>MGLKALFFDVQGTLVDFYSTITREGEAFSAVRGFQADWTTVTEQWRAEYRSRLDQVIKGERPWTTTDRIYREALDGILANHPWGASLNSADRDELNSLWSKLIPWDDTAPGLARLRSKYITSTLSNGSMASVLRISKLGALPFDAILTAELVRSSKPDPKVYQLALDSVGIEAHQAMMVACHKYDLQAAKRLGFKVAFIARPFEFGPNKKVDTKPEQYFDYYANSVVELAGMLGALEHHHHHH[2x]

Microbial epoxide hydrolases, cis-epoxysuccinate hydrolases (CESHs), have been utilized for commercial production of enantiomerically pure L(+)- and D(−)-tartaric acids for decades. All these three CESH[L]s exhibit high sequence identity (>60%) with L-2-haloacid dehalogenases, which are members of the haloacid dehalogenase (HAD)-like superfamily. Studies have shown that both RhCESH[L] and KlCESH[L] adopt a two-step catalytic reaction mechanism by 18O-labeling studies.

After crystal screening and optimization, crystal structures of RhCESH[L] and KlCESH[L] were successfully resolved at 1.94 Å and 2.02 Å, respectively. RhCESH[L] and NoCESH[L] share identical sequences, whereas KlCESH[L] displays only 36% sequence identity with RhCESH[L]. The core domains of both RhCESH[L] and KlCESH[L] can be well superimposed (with an r.s.m.d value of 0.944 Å), while there are some notable differences in the cap domain. Furthermore, residues from the core domain surrounding the catalytic pocket in KlCESH[L] can be superimposed well with those in RhCESH[L], while some significant conformational differences are observed in the residues from the cap domain. Furthermore, similar hydrophilic and hydrophobic interactions at the dimer interface are also observed in KlCESH[L]. Careful analysis of the obtained CESH[L] structures revealed a potential active catalytic triad consisting of D18, H190, and E212, along with the active water molecule in RhCESH[L] while the corresponding possible catalytic triad in KlCESH[L] consists of D48, H221, and E243.(3~{R},4~{S})-1-(4-fluorophenyl)-3-[(3~{S})-3-(4-fluorophenyl)-3-oxidanyl-propyl]-4-(4-hydroxyphenyl)azetidin-2-one 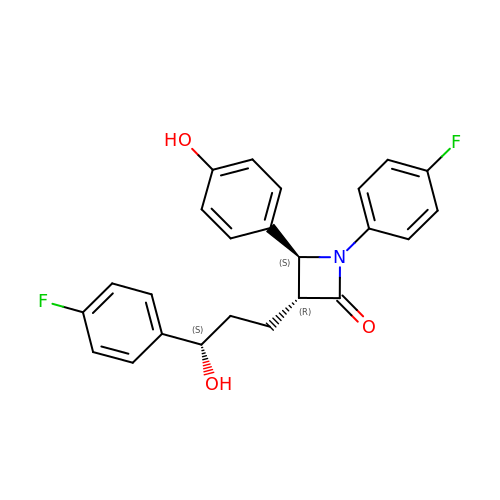| C24 H21 F2 N O3 | OLNTVTPDXPETLC-XPWALMASSA-N octyl sulfate | C8 H17 O4 S | 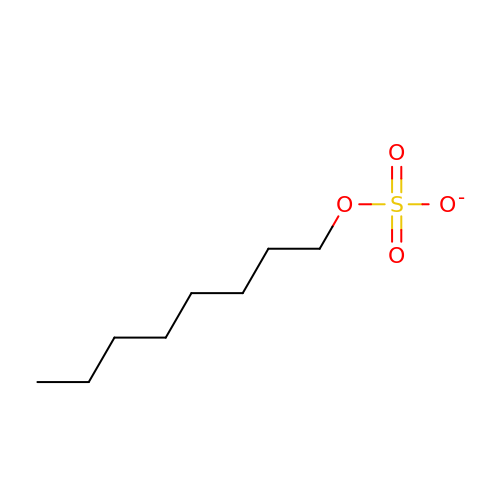UZZYXUGECOQHPU-UHFFFAOYSA-M4-nitrobutanoic acid | C4 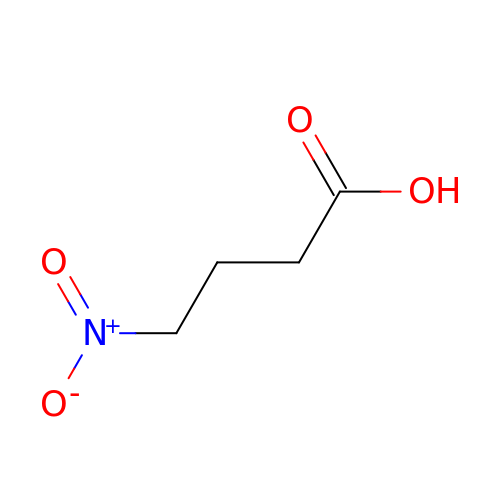H7 N O4 | SUFKNMKUIYHURJ-UHFFFAOYSA-N Toxigenic Vibrio cholerae causes disease by producing the primary virulence factors cholera toxin (CT) and the toxin coregulated pilus (TCP). Most AraC/XylS-family members, including ToxT and AraC, contain an N-terminal regulatory/dimerization domain and a C-terminal DNA-binding domain. We present here the crystal structures of the V. cholerae master virulence activator ToxT in both the UFA-bound and apo states. We have presented here the results of structural and functional studies of ToxT that reveal the detailed molecular basis for the regulation of virulence in V. cholerae by the UFA components of bile or synthetic ToxT inhibitors.

We solved the 1.8 Å resolution crystal structure of wild-type ToxT from V. cholerae serogroup O42 strain SCE-256 (ToxTENV256). The asymmetric unit is composed of a monomer of ToxTENV256 in a closed conformation. ToxTENV256 and ToxTEPI are superposable, with a root-mean-square deviation (RMSD) of 0.432 Å for 204 α-carbons. The N-terminal regulatory domain contains a nine sheet β-barrel with three α helices on one face. The C-terminal domain is entirely α-helical and contains two helix-turn-helix DNA-binding motifs. As with ToxTEPI, ToxTENV256 purified from E. coli with a UFA bound within the hydrophobic pocket inside the end of the regulatory domain β-barrel, at the interface between the regulatory domain and the DNA-binding domain. Tyr13, Lys32, and Lys231 in ToxTENV256 are analogous to Tyr12, Lys31, and Lys230 in ToxTEPI. When aligned to the structure of the AraC dimer, helix α3 of UFA-bound ToxT is at an angle that precludes dimerization. The recognition helix (α6) in the first helix-turn-helix motif in the DNA-binding domain of UFA-bound ToxT is turned perpendicular to the recognition helix in the second helix-turn-helix motif (α9), which prevents it from fitting within the major groove of DNA. These results suggest UFAs inhibit both dimerization and DNA-binding of ToxT by controlling the positions of α3 and α6, respectively.

> MRENNTSFLVNVYDLKKFDTYAFNKVFIDDYKIFWINKGSAKLVDKNCLVSYTITASSVVLLKKNSIQRFSLMSLSDESISVCVLTIKNKFVNSLRHYLQGDLMIRNLYNEKKDLLLWNCELNDISVLGEIVSTYDQTQYSEDFLKIFFSGFFSKVEKKYNSIFITDDLDAMEKISCLVKSDITRNWRWADICGELRTNRMILKKELESRGVKFRELINSIRISYSISLMKTGEFKIKQIAYQSGFASVSYFSTVFKSTMNVAPSEYLFMLTGVAEE(3alpha,8alpha)-cholest-5-ene-3,20-diol 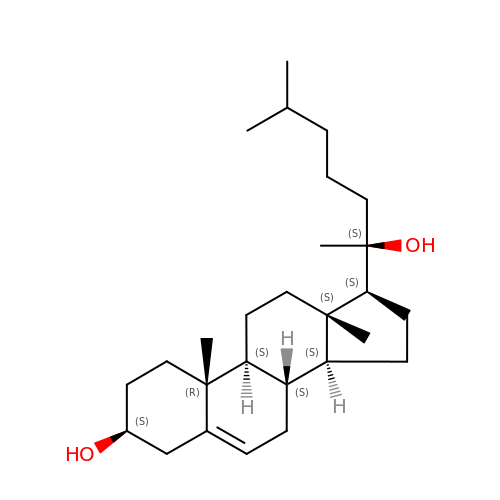| C27 H46 O2 | MCKLJFJEQRYRQT-APGJSSKUSA-N> MAKTLGLHILADLYGVDADK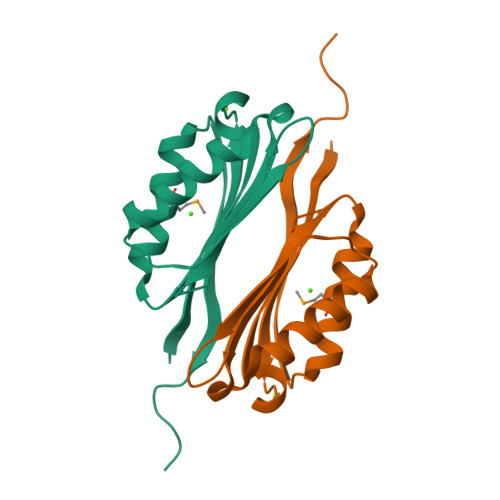IDRVEDIRELLEGAVKYANLTKISSHYYQFQPHGATGVVLLAESHISIHTWPEHGLATVDVYTCGDPSKAYRAMDYIITQLNPKRIDKQVHERGIVEEESNQSEAEKLRSILLQV>GAMGGGGYHLFNELAHSYDLHTPPENFQHDHAFV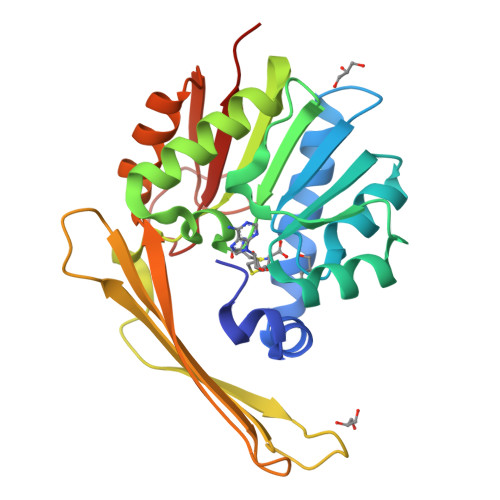LEEARSLGTPCRLLDVGCGTGALLEKARNAGILATGIDASPKMVELAQARVGQEAVTLRRMEEIDEEGAYDLVVSLCWTIHYSAGRAGLLDVLKRIHRALRPGGRGIIQIAHAAHAPKRTLESRIPGPNGEPDDVVMLFRFRPAPTEEPSMHAEYVYACKSLNELLYENHLLSMTDAHAFAACAREAGFAQVTVYDSSKRAPFSAAPNPLVCVEKAHDVGR[4x]>MAKDIGINSDPNSSSVDKLMKSSGVSNPTYTLVWKVWILAVTLYFAIRIPLTLVFPSLFSPLLPLDILASLALIADIPLDLAFESRRTSGRKPTLLAPSRLPDLLAALPLDLLVFALHLPSPLSLLSLVRLLKLISVQRSATRILSYRINPALLRLLSLVGFILLAAHGIACGWMSLQPPSENPAGTRYLSAFYWTITTLTTIGYGDITPSTPTQTVYTIVIELLGAAMYGLVIGNIASLVSKLDAAKLLHRERVERVTAFLSYKRISPELQRRIIEYFDYLWETRRGYEEREVLKELPHPLRLAVAMEIHGDVIEKVPLFKGAGEEFIRDIILHLEPVIYGPGEYIIRAGEMGSDVYFINR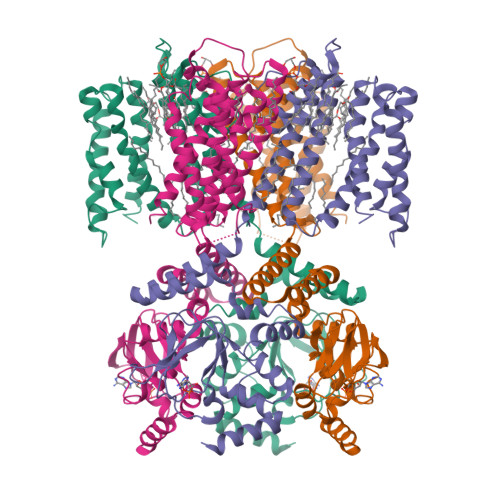GSVEVLSADEKTRYAILSEGQFFGEMALILRAPRTATVRARAFCDLYRLDKETFDRILSRYPEIAAQIQELAVRRKELESSGLVPRGSVKHHHH[4x]The double-ring AAA+ ATPase Pex1/Pex6 is required for peroxisomal receptor recycling and is essential for peroxisome formation. Pex1 and Pex6 are both composed of two N-terminal domains (N1 and N2) followed by two AAA cassettes, known as the D1 and D2 domains. Pex1/Pex6 is the only known double-ring heterohexamer of the type II AAA+ family, with both subunits capped by a unique pair of N-terminal domains. We used a Pex6 Walker B mutant (E832Q) and “trapped” the heterohexamer processing an endogenous substrate along the central channel formed by the active D2 ring.

In this conformation, the D1 ring is symmetric and all ATPase domains of the D1 ring are bound to ATP. The resulting central pore of the D1 ring has a diameter of approximately 15 Å. The substrate is threaded into a right-handed spiral staircase formed by pore loops 1 of Pex1(D2) and Pex6(D2). The pore loops 1 of chain A (Pex1) and E (Pex1) occupy the highest and the lowest position of the spiral (grey highlight in 3d). D2 of chain F (Pex6) does not directly contact the substrate and does not follow the spiral arrangement (“seam” subunit). We therefore define this conformation of the heterohexamer as the “single-seam” state. The aromatic residue (Pex1 F771; Pex6 Y805) and the isoleucine of the involved pore loops 1 bind to the substrate every two amino acids in a “forceps”-like manner. We therefore measured the buried surface area between adjacent protomers and distances between Walker A and arginine-fingers of the associated protomers. In line with these observations, our analysis suggests that both the “bottom” Pex1(D) and the disengaged “seam” Pex1(F) D2 domains are indeed in an ADP-bound state. In Pex1/Pex6 “single-seam” state, however, the D2 domains are organized as tight dimers and this signal is not passed on to the directly neighboring subunit, but two subunits further.

>[3x]TILKNGAIQLLKKVILRSTVCKMDFPKDNLFVVYISDGAQLPSQKGYASIVKCSLRQSKKSDSDNKSVGIPSKKIGVFIKCDSQIPENHIALSSHLWDAFFTHPMNGAKIKLEFLQMNQANIISGRNATVNIKYFGKDVPTKSGDQYSKLLGGSLLTNNLILPTEQIIIEIKKGESEQQLCNLNEISNESVQWKVTQMGKEEVKDIIERHLPKHYHVKETGEVSRTSKDEDDFITVNSIKKEMVNYLTSPIIATPAIILDGKQGIGKTRLLKELINEVEKDHHIFVKYADCETLHETSNLDKTQKLIMEWCSFCYWYGPSLIVLDNVEALFGKPQANDGDPSNNGQWDNASKLLNFFINQVTKIFNKDNKRIRVLFSGKQKTQINPLLFDKHFVSETWSLRAPDKHARAKLLEYFFSKNQIMKLNRDLQFSDLSLETEGFSPLDLEIFTEKIFYDLQLERDCDNVVTRELFSKSLSAFTPSALRGVKLTKETNIKWGDIGALANAKDVLLETLEWPTKYEPIFVNCPLRLRSGILLYGYPGCGKTLLASAVAQQCGLNFISVKGPEILNKFIGASEQNIRELFERAQSVKPCILFFDEFDSIAPKRGHDSTGVTDRVVNQLLTQMDGAEGLDGVYILAATSRPDLIDSALLRPGRLDKSVICNIPTESERLDILQAIVNSKDKDTGQKKFALEKNADLKLIAEKTAGFSGADLQGLCYNAYLKSVHRWLSAADQSEVVPGNDNIEYFSINEHGRREENRLRLKTLLQQDVVHETKTSTSAASELTAVVTINDLLEACQETKPSISTSELVKLRGIYDRFQKDR;>MKASLTFSLSGIYAPCSISRDIYLEYGDKKAECLYGTIRLPQYGPGCTPGKIVHCVLDDSLPFCSIVVPSKLFGFMPTQPTMDFCYFEPILDNVVPVLDSVTFLINEQLYSKLMDLPQEMQQIQFLHYKYNINSMETVVHSRDILTSGLCQILNCSPFPQGLVDFTETQLILVNDTEQKLSALKYANEDEEYALPKIGTNSALSIDLESLPCTISRDLLRPAPHINDDNSIYAFTDAETLLRLDVTSGSFITVSNMGCVRLVKLFVLLLPNGFKKRTIYAPPKIIASFPDCSVVTISKSNIGHTDIPIANQVFISRVGGWLQSQKCFQNIILTTLKKFFSESKRILCQNDLIPIAFDSSMADLNIAEENDESDDEDELGQYYKNDSLVWFFVTSAELDCFSKDNSHFIIDPNRTKLITTNITNRRPLPLSRSNLQRYYGFAETFYYDLHIFPYVRQLVNILETSFNCSQRGITLNASVLLHSTTNNVGKATMVRFASKYLGIHLLEIDCLSLTSNSRQLDSTSKIIGYIRAKCENVLPYASPAVIFLAHLDSILLDVNANQDPEAIKLQKSINFEMSKLLDDFTFKFPGTTFVGSVNNIDNVPSSFRSHMRFEILVPVPSEAQRLRIFQWYLSSHELNRDVQQKVPVSYMDNISFSSLSSYSAGLTPLDIKSIVETARMTATARFYQESKKCGWLPQSILITQEDLSKATSKARNEFSVSIGAPQIPNVTWDDIGGIDFVKGEILDTIDMPLKHPELFTSGMKKRSGILFYGPPGTGKTLMAKAIATNFSLNFFSVKGPELLNMYIGESEANVRRVFQKAREAKPCVIFFDQIDSVAPKRGNQGDSGGVMDRIVSQLLAELDGMSTDADGVFVIGATNRPDLLDEALLRPGRFDKLLYLGIPDTDTKQLNILEALTRKFVLDNDVKLIELAKLCPFNYTGADFYALCSDAMLNAMSRIARMVEKKVSQHNELTGENISTRRWFDKIATKEDTKVVVKMEDFLKAQEQLTPSVSRAELNHYEAVRANFEGA[3x]> MTKRAVLAGGCFWGMQDLIRKLPGVIETRVGYTGGDVPNATYRNHGTHAEGIEIIFDPERISYRRILELFFQIHDPTTKDRQGNDIGTSYRSAIYYVDDEQKRIAQETIADVEASGLWPGKVVTEVEP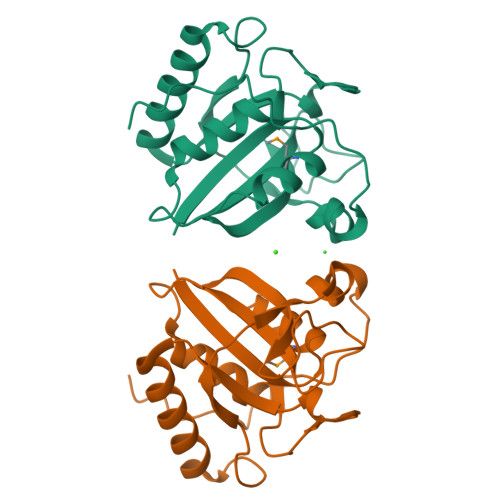VRDFWEAEPEHQNYLERYPNGYTCHFPRPNWVLPRRSAAE>MAELACFCYPHLENDSYKFIPFNNLAIKAMLTAKVDKK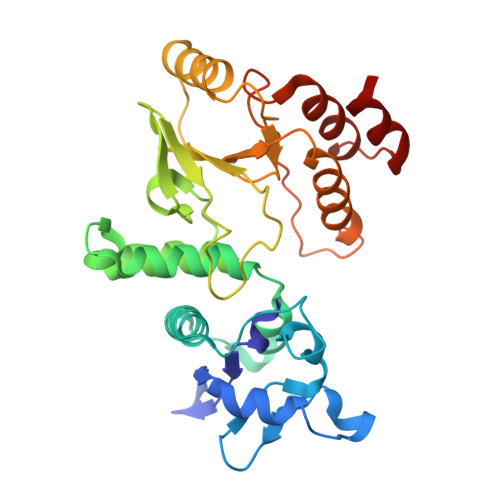DMDKFYDSIIYGIAPPPQFKKRYNTNDNSRGMNFETIMFTKVAMLICEALNSLKVTQANVSNVLSRVVSIRHLENLVIRKENPQDILFHSKDLLLKSTLIAIGQSKEIETTITAEGGEIVFQNAAFTMWKLTYLEHQLMPILDQNFIEYKVTLNEDKPISDVHVKELVAELRWQYNKFAVITHGKGHYRIVKYSSVANHADRVYATFKSNVKTGVNNDFNLLDQRIIWQNWYAFTSSMKQGNTLDVCKRLLFQKMK[10x]> GPSQVIFNSVEKFYIPGGDVTCHYTFTQHFIPRRKDWIGIFRVGWKTTREYYTFMWVTLPIDLNNKSAKQQEVQFKAYYLPKDDEYYQFCYVDEDGVVRGASIPFQFRPENEEDILVVTTQGE;> GPMPPPQKIPSVRPFKQRKSLAIRQEEVAGIRAKFPNKIPVVVERYPRETFLPPLDKTKFLVPQELTMTQFLSIIRSRMVLRATEAFYLLVNNKSLVSMSATMAEIYRDYKDEDGFVYMTYASQETFG

Autophagy receptors target cargo to autophagy by binding ATG8 on autophagosomal membranes. In this study we discovered that the ubiquitin-binding autophagy receptor NDP52 binds preferentially to LC3C, in contrast to other autophagy adaptors including p62 and NBR1 that nonselectively interact with several human ATG8 orthologs. NDP52 comprises an N-terminal SKICH domain of unknown structure (aa 1–127), a central coiled-coil forming region (aa 140–420) and a C-terminal ubiquitin-binding Zn finger domain (ZnF, aa 421–446). We determined the crystal structure of the NDP52 N terminus (aa 21–141) containing the SKICH domain and CLIR in isolation and in complex with LC3C.

The NDP52 CLIR was disordered in crystals of apo-NDP52 but became structured in the 2.5 Å complex structure of NDP52 bound to LC3C. Similar to other LC3-LIR complexes (Noda et al., 2010) and to SUMO-SIM interactions (Hecker et al., 2006), the CLIR forms a short β strand that fits into the canonical, hydrophobic LIR binding groove of LC3C. As expected from the NMR data and mutational analysis, the interaction is driven by extensive hydrophobic interactions of Leu134, Val135, and Val136. Ile133 of the NDP52 CLIR β strand is at the Trp340-equivalent position but due to its shorter side chain does not occupy the aromatic pocket and is therefore largely solvent exposed. And in contrast to canonical LIR β strands where the first and fourth residue mediate binding, the CLIR-LC3C interaction is dependent on three consecutive hydrophobic residues, the Leu-Val-Val motif, which occupy position two, three, and four of the CLIR β strand. Val136 in position four and Leu134 in position two of the CLIR β strand cooperate to occupy a complementary, smooth hydrophobic surface on LC3C in which the Leu-pocket is less pronounced than in other ATG8 family members. In addition, Val135 on the opposite face of the β strand exploits another hydrophobic wall of the LC3C binding pocket, formed by Phe33. However, it also improves shape complementarity with the hydrophobic CLIR pocket, and enables additional interstrand hydrogen bonds between the CLIR of NDP52 and the β2-strand of LC3C. While the LIR of p62 forms three backbone hydrogen bonds with the β2-strand of LC3B, five bonds are formed between the CLIR and LC3C, which may partly compensate for the missing aromatic-pocket interactions. The N-terminal α1 helix of LC3C is disordered in our structure; it is possible that this helix is stabilized by acidic residues upstream of canonical LIRs (Noda et al., 2010).>[2x]MAHHHHHHSSGLEVLFQGPMSNDVAELKQYVLAHVSAQNASADGVLARIDDDGDGPRSWTTQWIRAGEEREQAGDLLAATTFYNLARFPFVDSPGRAE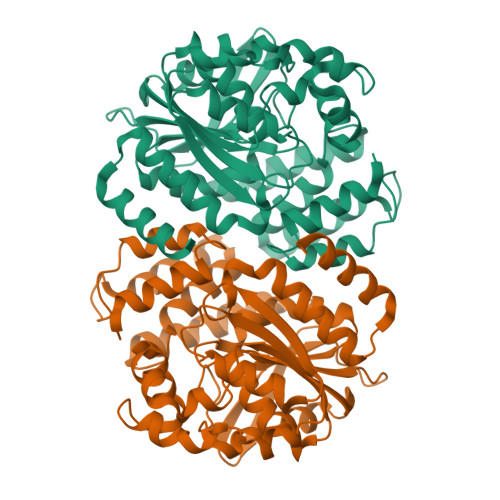ALRRCVAVFDRWRRTVPGIERLELRLPGGVVRAWAAGLSTTERRPVLLMTGGIVSIKEQWAPILPELARYGFAAVVTELPGVGENELRYDLDSAALFGVLLDAVAERADTSRAYALALSFSGHLALRAAPSEPRLRGIVTAGAPVAAFFTDKEWQAAVPRVTVDTLARLTQTTPATVFDHVRNWALTPQDLAGVRIPVAYVASGRDEIIPPADPALLRTHVRDFRTITHDDVHGSPAHFPHTRLWTLAQVLEMSGADPRHRAAVDGALAQVEGGRA> MKLRMSRQDIRD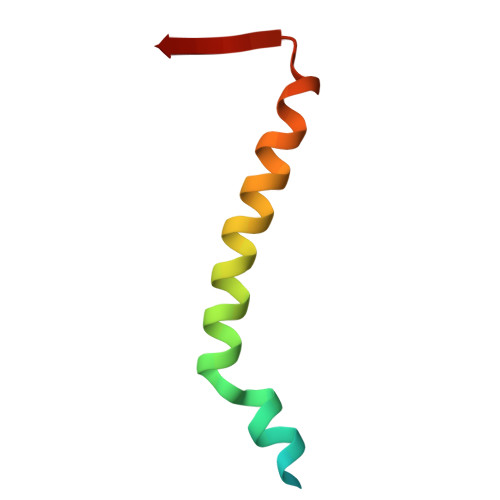EFKESEGDPHVKGKIRQMQRAAAQRRMMEDVPKADVIVTN>MISGWGARPEEQYEMIRAAVPPSEAEPRLQEALVVVNALLPAPITLDDALGSLDDTRRLVKARALARTYHACMVNLERLARHHPGLEAPTIDGAVAAHQDKMRRLADTCMATILQMYMSVGAADKSADVLVSQAIR[4x];>[4x]MAAATADDEGSAATILKQAIAGDRSLVEAAEAISQQTLLRLACEVRQVGDRQPRFTATSIARVDVAPGCRLRFVLDGSPEDAYVTSEDYFKRCCGQSSYRGFAVAVLTANEDHVHSLAVPPLVLLHRFSLFNPRDLLDFELACLLMYLENCPRSHATPSTFAKVLAWLGVAGRRTSPFERVRCLFLRSCHWVLNTLMFMVHVKPFDDEFVLPHWYMARYLLANNPPPVLSALFCATPTSSSFRLPGPPPRSDCVAYNPAGIMGSCWASEEVRAPLVYWWLSETPKRQTSSLFYQFCGSLEVLFQ

HSV-1 tegument proteins pUL7 and pUL51 promote virus assembly by stimulating the cytoplasmic wrapping of nascent virions. pUL7 and pUL51 form a complex that co-localizes with Golgi markers both during infection and when co-transfected into cells, palmitoylation of residue Cys9 being required for pUL51 membrane association. We characterized the pUL7:pUL51 complex by solution scattering and solved the atomic-resolution structure of the proteolysis-resistant core of this complex using X-ray crystallography. pUL7 comprises a single globular domain that binds one molecule of pUL51 via a hydrophobic surface, a second molecule of pUL51 being recruited to the solution complex via the N-terminal region of pUL51. While the fold of pUL7 is not similar to any known structure, the α-helical pUL51 protein shares unanticipated structural similarity to components of the ESCRT-III membrane-remodeling machinery. Given the conservation of the pUL7:pUL51 interaction, the conserved localization of this complex to trans-Golgi membranes, and the established evidence supporting roles for pUL7 or pUL51 homologues in virus assembly, we propose that pUL7 and pUL51 form a complex that is conserved across herpesviruses and functions to promote virus assembly by stimulating cytoplasmic envelopment of nascent virions.

The pUL7:pUL51(8–142) complex was crystallized and its structure was solved by four-wavelength anomalous dispersion analysis of a mercury acetate derivative. The structure of native pUL7:pUL51(8–142) was refined to 1.83 Å resolution with residuals R = 0.195, Rfree = 0.220 and excellent stereochemistry, 99% of residues occupying the most favored region of the Ramachandran plot (Supplementary file 1–Table S2). Strikingly, the molecules of pUL7 and pUL51 in the structure were arranged as a hetero-octamer, with single β-strands from each pUL7 and pUL51 molecule in the asymmetric unit forming a central β-barrel. Closer inspection revealed that the pUL7 strands in this β-barrel comprised the C-terminal amino acids encoded by the restriction site and from the human rhinovirus 3C protease recognition sequence that remained following proteolytic removal of the GST purification tag. We therefore suspected that this hetero-octameric pUL7:pUL51 arrangement was an artefact of crystallization. Taken together, these results suggest that pUL7 and pUL51 residues 41–142 assemble to form a heterodimeric ‘core’ complex and that recruitment of the additional pUL51 molecule in the native heterotrimeric complex is mediated by the N-terminal region (residues 8–40) of pUL51. Structure-based searches of the Protein Data Bank did not reveal any other domains with a similar fold, which we will henceforth refer to as the Conserved UL7(Seven) Tegument Assembly/Release Domain (CUSTARD) fold. pUL51 comprises a hydrophobic loop region followed by a helix-turn-helix.> GSHMALDLTGYLDRINYRGATDPTLDVLRDLVSAHTGAIAFENLDPLMGVPVDDLSAEALADKLVDRRRGGYCYEHNGLIGYVLAELGYRVRRLAGRVVWLAPPDAPTPAQTHTVLAVTFPGCQGPYLVDVGFGGMTPTAPLRLETGTVQQTALEPYRLDDRGDGLVLQAMVRDEWQALYEFSTLTRPQVDLRVGSWFVSTHPTSHFVTGLMAATVADDARWNLMGRNLAIHRRGGTEKILLEDAAAVVDTLGDRFGINVADVGERGRLEARIDKVCFGAENR

NAT is a cytosolic enzyme that is found in M. tuberculosis and many other organisms. This enzyme catalyses the transfer of an acyl group, usually an acetyl, to an arylamine substrate using a conserved cysteine residue by a Ping-Pong bi-bi mechanism. NAT utilises Pr-CoA in addition to acetyl-CoA (Ac-CoA) as an acyl donor, both of which are products of degradation of the alkyl moiety of cholesterol. Arylamine N-acetyltransferase is one of the novel targets that plays an important role in cell wall synthesis and intracellular survival of mycobacteria within the macrophage.

To validate the observations obtained using MS, the 3D-structure of MMNAT was determined in complex with compound 1, the parent piperidinol identified from the HTS. The crystallographic structure determination was performed by incubating MMNAT with 1 in solution (15∶1 inhibitor to protein ratio in the native form) and then to crystallise it (co-crystallisation). According to the proposed mechanism of inhibition, this method is expected to allow time for the ligand to mature into the covalent modification of the active site cysteine with the 3-phenyl-3-oxopropyl moiety (POP). The crystals diffracted to 2.7 Å and data were processed as described in Methods and in Table S2. Upon refinement of the co-crystallised complex MMNAT-POP, a continuous excess electron density connected to the active site Cys70 was observed, consistent with the proposed 3-phenyl-3-oxopropyl modification. The binding site of the fragment which was observed attached to the active site cysteine was accommodated by the fragment predicted from the MS studies using a 1∶1 ratio of compound 1 to MMNAT. These data are entirely compatible with the MS data obtained using the same compound to MMNAT ratio, since the protein remains in the native state throughout the crystallisation and excess inhibitor was removed by buffer exchange prior to crystallisation as described in Methods. Therefore, we propose that in the presence of an equimolar amount of the inhibitor, the active site cysteine Cys70 is the residue which is modified. The mechanism of inactivation of NAT involves the formation of PVKs that form an adduct with the active site cysteine. Extensive dialysis of the enzyme after incubation with compound 1 was completely ineffective in restoring the activity of the enzyme, supporting the proposal of tight irreversible binding of 1 to the NAT enzyme.> MTSGSALFDTNILIDLFSGRREAKQALEAWPPQNAISLITWMEVMVGAKKYHQEQR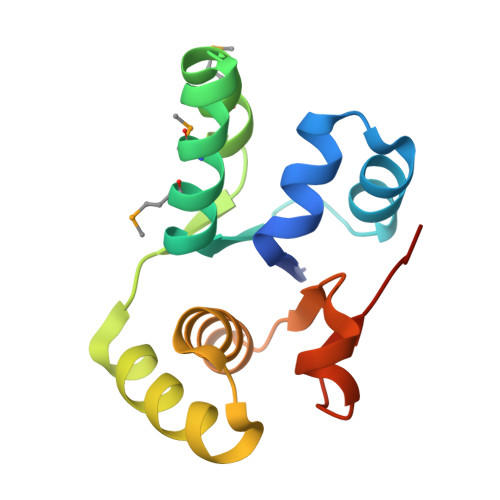TRMALSTFNIINISQDIAERSVALRQEYKLKLPDAIILATAQLHRLELITRNTKDFAGIPGVVTPYEIHPE> GPASQHFLSTSVQGPWERAISPNKVPYYINHETQTTCWDHPKMTELYQSLADLNNVRFSA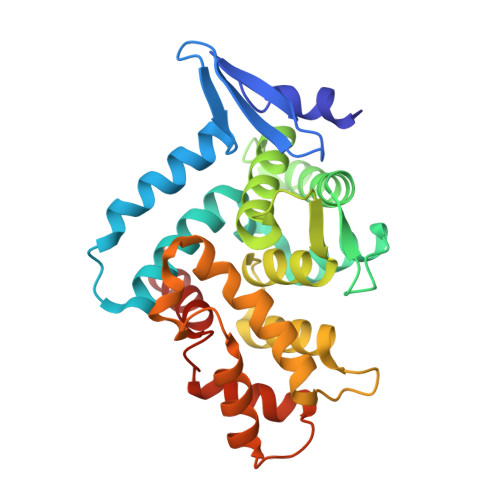YRTAMKLRRLQKALCLDLLSLSAACDALDQHNLKQNDQPMDILQIINCLTTIYDRLEQEHNNLVNVPLCVDMCLNWLLNVYDTGRTGRIRVLSFKTGIISLCKAHLEDKYRYLFKQVASSTGFCDQRRLGLLLHDSIQIPRQLGEVASFGGSNIEPSVRSCFQFANNKPEIEAALFLDWMRLEPQSMVWLPVLHRVAAAET>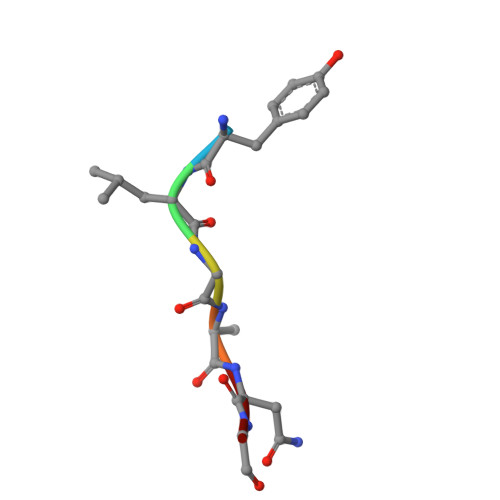 YLGANG>MDRASELLFYVNGRKVIEKNVDPETMLLPYLRKKLRLTGTKYGCGGGGCGACTVMISRYNPITKRIRHHPANACLIPICSLYGAAVTTVEGIGSTHTRIHPVQERIAKCHGTQCGFCTPGMVMSIYTLLRNHPEPTLDQLTDALGGNLCRCTGYRPIIDACKTFCKTSGCCQSKENGVCCLDQGINGLPEFEEGSKTSPKLFAEEEFLPLDPTQELIFPPELMIMAEKQSQRTRVFGSERMMWFSPVTLKELLEFKFKYPQAPVIMGNTSVGPEVKFKGVFHPVIISPDRIEELSVVNHAYNGLTLGAGLSLAQVKDILADVVQKLPEEKTQMYHALLKHLGTLAGSQIRNMASLGGHIISRHPDSDLNPILAVGNCTLNLLSKEGKRQIPLNEQFLSKCPNADLKPQEILVSVNIPYSRKWEFVSAFRQAQRQENALAIVNSGMRVFFGEGDGIIRELCISYGGVGPATICAKNSCQKLIGRHWNEQMLDIACRLILNEVSLLGSAPGGKVEFKRTLIISFLFKFYLEVSQILKKMDPVHYPSLADKYESALEDLHSKHHCSTLKYQNIGPKQHPEDPIGHPIMHLSGVKHATGEAIYCDDMPLVDQELFLTFVTSSRAHAKIVSIDLSEALSMPGVVDIMTAEHLSDVNSFCFFTEAEKFLATDKVFCVGQLVCAVLADSEVQAKRAAKRVKIVYQDLEPLILTIEESIQHNSSFKPERKLEYGNVDEAFKVVDQILEGEIHMGGQEHFYMETQSMLVVPKGEDQEMDVYVSTQFPKYIQDIVASTLKLPANKVMCHVRRVGGAFGGKVLKTGIIAAVTAFAANKHGRAVRCVLERGEDMLITGGRHPYLGKYKAGFMNDGRILALDMEHYSNAGASLDESLFVIEMGLLKMDNAYKFPNLRCRGWACRTNLPSNTAFRGFGFPQAALITESCITEVAAKCGLSPEKVRIINMYKEIDQTPYKQEINAKNLIQCWRECMAMSSYSLRKVAVEKFNAENYWKKKGLAMVPLKFPVGLGSRAAGQAAALVHIYLDGSVLVTHGGIEMGQGVHTKMIQVVSRELRMPMSNVHLRGTSTETVPNANISGGSVVADLNGLAVKDACQTLLKRLEPIISKNPKGTWKDWAQTAFDESINLSAVGYFRGYESDMNWEKGEGQPFEYFVYGAACSEVEIDCLTGDHKNIRTDIVMDVGCSINPAIDIGQIEGAFIQGMGLYTIEELNYSPQGILHTRGPDQYKIPAICDMPTELHIALLPPSQNSNTLYSSKGLGESGVFLGCSVFFAIHDAVSAAR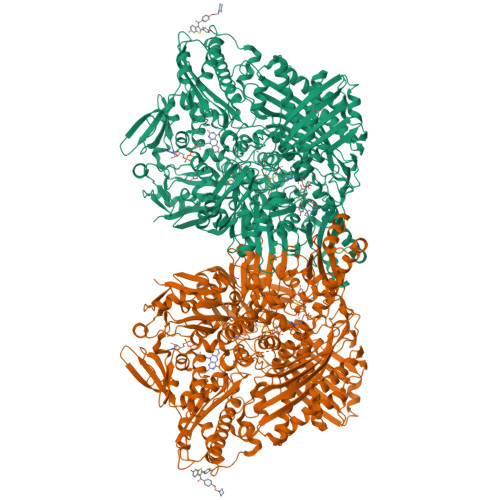QERGLHGPLTLNSPLTPEKIRMACEDKFTKMIPRDEPGSYVPWNVPI[2x]> TTIVSVRRNGHVVIAGDGQATLGNTVMKGNVKKVRRLYNDKVIAGFAGGTADAFTLFELFERKLEMHQGHLVKAAVELAKDWRTDRMLRKLEALLAVADETASLIITGNGDVVQPENDLIAIGSGGPYAQAAARALLE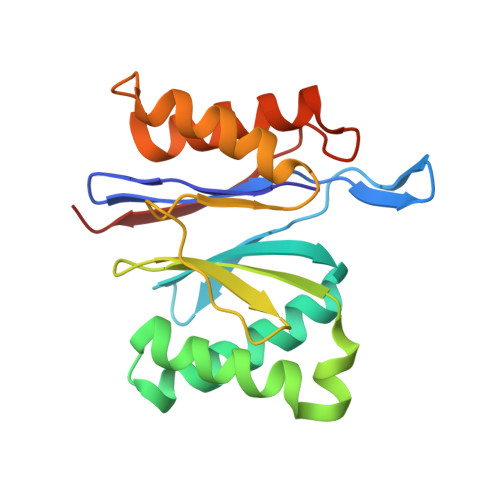NTELSAREIAEKALDIAGDICIYTNHFHTIEELSYKA We describe here the use of an artificial cofactor employing the well‐known biotin‐streptavidin system to catalyze a Baylis‐Hillman reaction. As protein host, we chose streptavidin, as it can be easily crystallized and thereby supports the design process. There are several examples using streptavidin as the host for these cofactors, since its natural ligand biotin binds strongly (K d∼10−15 M) and is easy to modify with catalysts at the carboxylic acid group. No enzyme is known to naturally catalyze the Baylis‐Hillman reaction, a very versatile and atom‐economic C−C bond forming reaction for the production of various functionalized compounds and intermediates of active pharmaceutical ingredients (APIs).

We chose a derivative of DMAP as the artificial cofactor due to its low steric demand, which will facilitate its inclusion into the protein scaffold. The protein host around the cofactor was rationally designed on the basis of high‐resolution crystal structures obtained after each variation of the amino acid sequence. The location of the catalyst is in a shallow cavity at the surface of the protein. The system was evolved through repeated cycles of mutagenesis, activity tests, and structure determination. According to the presented structures and calculations the catalytically active site is too shallow to undergo interactions with 1.

>[2x]MASMTGGQQMGRDEAGITGTWYNQLGSTFIVTAGADGALTGTYESAAGKAESRYVLTGRYDSAPATDGSGTALGWTVAWKNNYRNAHSATTWSGQYVGGAEARINTQWLLTAGTTEANGWASTLVGHDTFTKVKPSAASIDAAKKAGVNNGNPLDAVQQ>MQRLFLLVAVMLLSGCLTAPPKEAARPTLMPRAQSYKDLTHLPAPTGKIFVSVYNIQDETGQFKPYPASNFSTAVPQSATAMLVTALKDSRWFIPLERQGLQN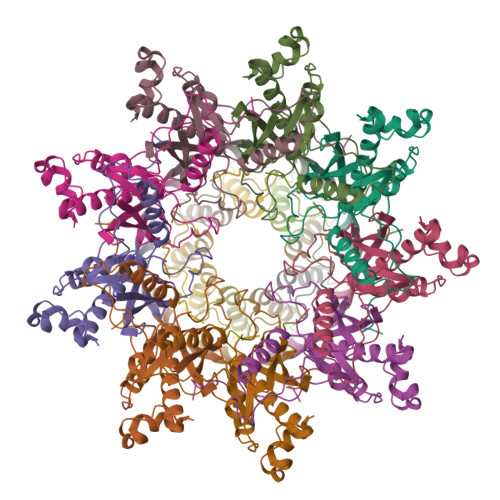LLNERKIIRAAQENGTVAINNRIPLQSLTAANIMVEGSIIGYESNVKSGGVGARYFGIGADTQYQLDQIAVNLRVVNVSTGEILSSVNTSKTILSYEVQAGVFRFIDYQRLLEGEVGYTSNEPVMLCLMSAIETGVIFLINDGIDRGLWDLQNKAERQNDILVKYRHMSVPPES[9x];>[9x]MRVKHAVVLLMLISPLSWAGTMTFQFRNPNFGGNPNNGAFLLNSAQAQNSYKDPSYNDDFGIETPSALDNFTQAIQSQILGGLLSNINTGKPGRMVTNDYIVDIANRDGQLQLNVTDRKTGQTSTIQVSGLQNNSTDF> MDRKDRLSEPPTLALRLKPYKTAIQQLRSVIRALKENTTVTFLPTPSLILQTVRSHCVSKITFNSSCLYITDKSFQPKTINNSTPLLGNFMYLTSSKDLTKFYVQDISDLSAKISMCAPDFNMEFSSACVHGQDIVRESENSAVHVDLDFGVVADLLKWIGPHTRVKRNVKKAPCPTGTVQILV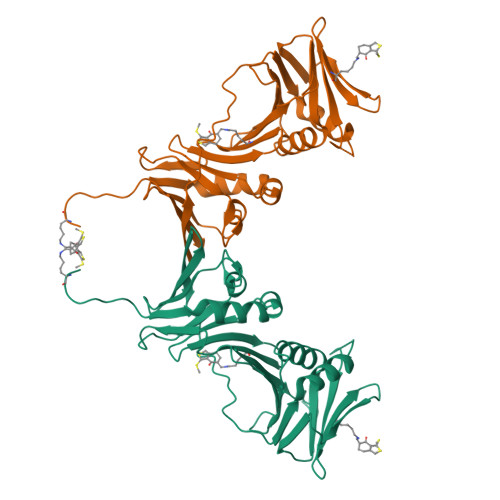HAGPPAIKFILTNGSELEFTSNNRVSFHGVKNMRINVQLKNFYQTLLNCAVTKLPCTLRIVTEHDTLLYVASRNGLFAVENFLTEEPFQRGDPFDKNYVGNSGKSR> MKDLVDTTEMYLRTIYELEEEGVTPLRARIAERLEQSGPTVSQTVARMERDGLVVVASDRSLQMTPTGRTLATAVMRKARLAERLLTDIIGLDINKVHDEACRWEHVMSDEVERRLVKVLKDVSRSPFGN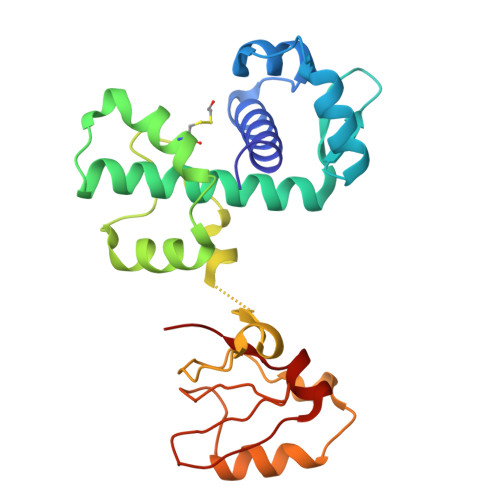PIPGLDELGVGNSDAAAPGTRVIDAATSMPRKVRIVQINEIFQVETDQFTQLLDADIRVGSEVEIVDRDGHITLSHNGKDVELLDDLAHTIRIEEL> MTDFYTIKDAQADLAIAPLNLTVLLAPYSTTPATTLESPTDGSLAIPPGYKSVGHFEKQAGLTLGNEFDSKDIEAYGEPEPIRTIINKRTTTFDFAMYQNQRNVLELIWTQDFSNIQPSEFGGIV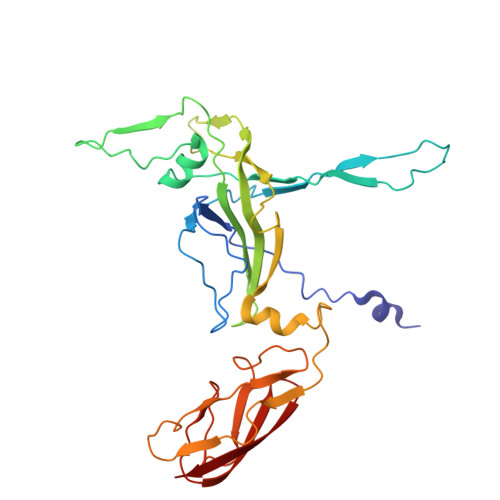LEAPKVPKNIYYRAILVGMDDRNDRPIWLYWLMPKVKLDKLDNQTLNDDNVIEYKPTLKAFRDDVVGYSVAQGFAGPGWRDLVATAGFGEALTALTITPGSPTVTVATGASHTAQLLVEGDNGINYTPDVVFTSSAPDKASVSAAGLVTGVAAGSATITATKGALTATATVTVTA(3Z)-N-(3-CHLOROPHENYL)-3-({3,5-DIMETHYL-4-[(4-METHYLPIPERAZIN-1-YL)CARBONYL]-1H-PYRROL-2-YL}METHYLENE)-N-METHYL-2-OXOINDOLINE-5-SULFONAMIDE | C28 H30 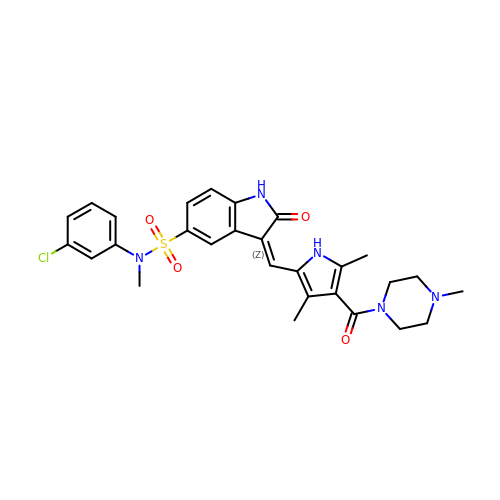Cl N5 O4 S | FPYJSJDOHRDAMT-KQWNVCNZSA-N>[2x]MIENLRNIAIIAHVDHGKTTLVDKLLQQSGTFDARAETQERVMDSNDLEKERGITILAKNTAIKWNDYRINIVDTPGHADFGGEVERVMSMVDSVLLVVDAFDGPMPQTRFVTKKAFAHGLKPIVVINKVDRPGARPDWVVDQVFDLFVNLDATDEQLDFPIIYASAL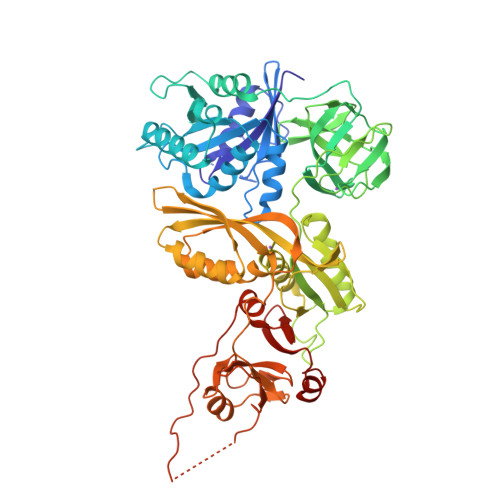NGIAGLDHEDMAEDMTPLYQAIVDHVPAPDVDLDGPLQMQISQLDYNNYVGVIGIGRIKRGKVKPNQQVTIIDSEGKTRNAKVGKVLTHLGLERIDSNIAEAGDIIAITGLGELNISDTICDPQNVEALPALSVDEPTVSMFFCVNTSPFCGKEGKFVTSRQILDRLNKELVHNVALRVEETEDADAFRVSGRGELHLSVLIENMRREGFELAVSRPKVIFREIDGRKQEPYENVTLDVEEQHQGSVMQALGERKGDLKNMNPDGKGRVRLDYVIPSRGLIGFRSEFMTMTSGTGLLYSTFSHYDDIRPGEVGQRQNGVLISNGQGKAVAFALFGLQDRGKLFLGHGAEVYEGQIIGIHSRSNDLTVNCLTGKKLTNMRASGTDEAVILVPPIKMSLEQALEFIDDDELVEVTPTSIRIRKRHLTENDRRRANRGQKEE>MTREEIKMIQKSWLRVIDKMDEAGLLFYRRLFDVEPKVRPLFKIDIEKQGRKLMDVLNWIVLNLQDIDAALDAARELARRHVKYGVKAEHYPVVGHTLIWTLRKMIGSEWTKQLEQ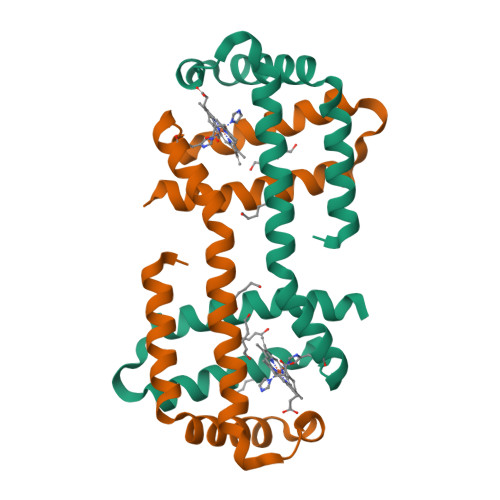LWTQAYEALAQVMIEEHHHHHH[2x]>[3x]LGSPMAYFVENFWGEKNSGFDVLYHNMKHGQISTKELADFVRERATIEEAYSRSMTKLAKSASNYSQLGTFAPVWDVFKTSTEKLANCHLDLVRKLQELIKEVQKYGEEQVKSHKKTKEEVAGTLEAVQTIQSITQALQKSKENYNAKCVEQERL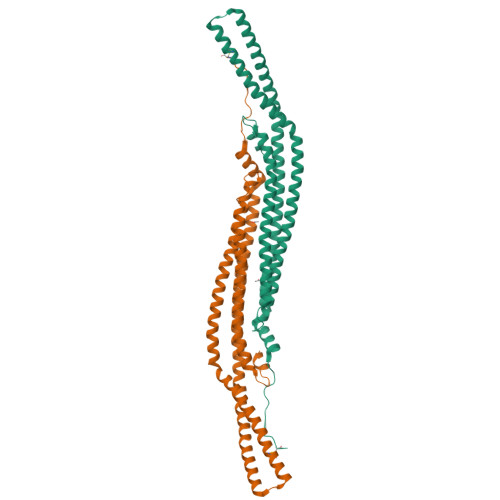KKEGATQREIEKAAVKSKKATDTYKLYVEKYALAKADFEQKMTETAQKFQDIEETHLIHIKEIIGSLSNAIKEIHLQIGQVHEEFINNMANTTVESLIQKFAESKGTGKERPGLIEFEECD>[3x]MGSSHHHHHHSQDPSQFIRRDIAQTVNGSLTLTQQTNLSAPLVSSSTGEFGGSLAANRTFTIRNTGAPTSIVFEKGPASGANPAQSMSIRVWGNQFGGGSDTTRSTVFEVGDDTSHHFYSQRNKDGNIAFNINGTVMPININASGLMNVNGTATFGRSVTANGEFISKSANAFRAIN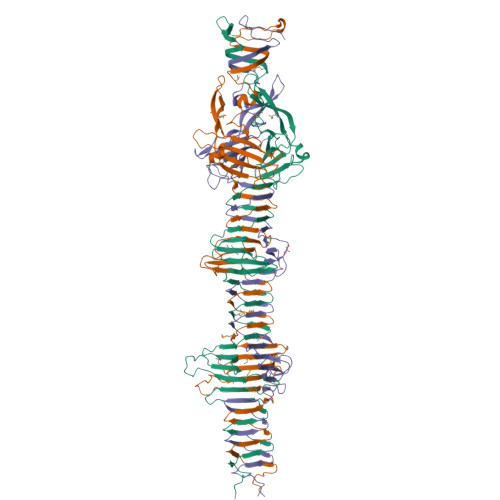GDYGFFIRNDASNTYFLLTAAGDQTGGFNGLRPLLINNQSGQITIGEGLIIAKGVTINSGGLTVNSRIRSQGTKTSDLYTRAPTSDTVGFWSIDINDSATYNQFPGYFKMVEKTNEVTGLPYLERGEEVKSPGTLTQFGNTLDSLYQDWITYPTTPEARTTRWTRTWQKTKNSWSSFVQVFDGGNPPQPSDIGALPSDNATMGNLTIRDFLRIGNVRIVPDPVNKTVKFEWVE> MDEATWERMWKHVAKIHPDGEKVAQRIRGATDLPKIPIPSVPTFQPSTPVPERLEAVQRYIRELQYNHTGTQFFEIKKSRPLTGLMDLAKEMTKEALPIKCLEAVILGIYLTNSMPTLERFPISFKTYFSGNYFRHIVLGVNFAGRYGALGMSRREDLMYKPPAFRTLSELVLDFEAAYGRCWHVLKKVKLGQSV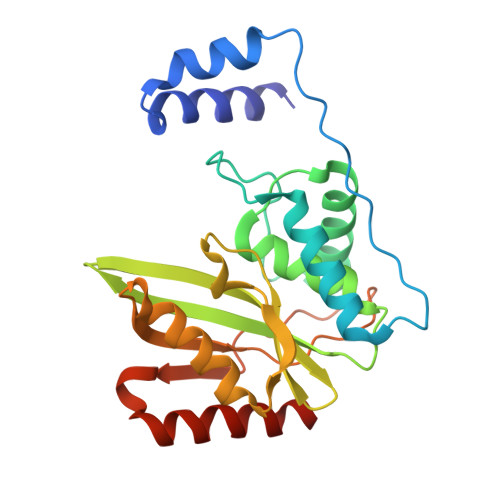SHDPHSVEQIEWKHSVLDVERLGRDDFRKELERHARDMRLKIG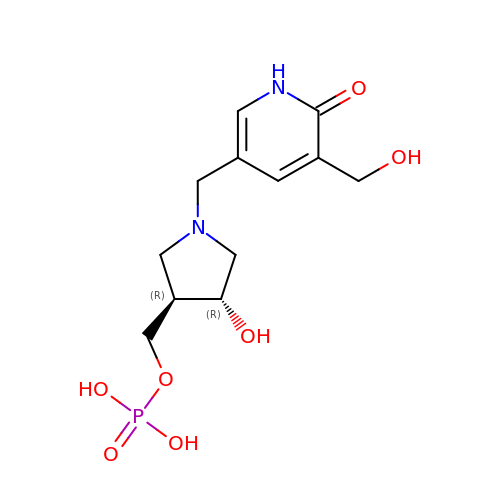[(3R,4R)-4-hydroxy-1-{[5-(hydroxymethyl)-6-oxo-1,6-dihydropyridin-3-yl]methyl}pyrrolidin-3-yl]methyl dihydrogen phosphate | C12 H19 N2 O7 P | SCJDKIAFOJPYRJ-MNOVXSKESA-N>[2x]GFREMPGGPVWRKHYITYRINNYTPDMNREDVDYAIRKAFQVWSN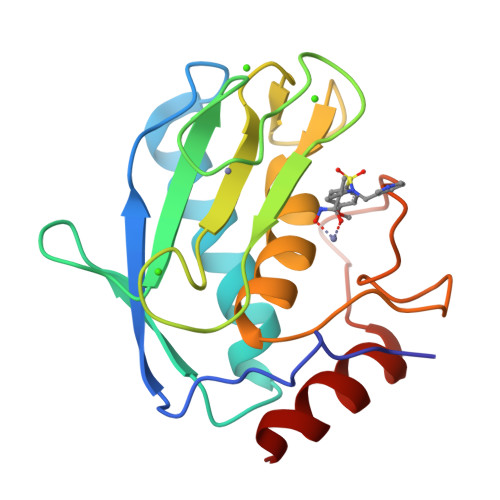VTPLKFSKINTGMADILVVFARGAHGDFHAFDGKGGILAHAFGPGSGIGGDAHFDEDEFWTTHSGGTNLFLTAVHEIGHSLGLGHSSDPKAVMFPTYKYVDINTFRLSADDIRGIQSLYGD> MFQKFISKHNAPINSTQLAATKTPAVAAPVLSVPNLSRSTILINATTTAVTTHSGLCHVVRIDETNPTNHHALSIAGSLSNVPADMIAFAIRFEVADGVVPTAVPALYDVYPIETFNNGKAISF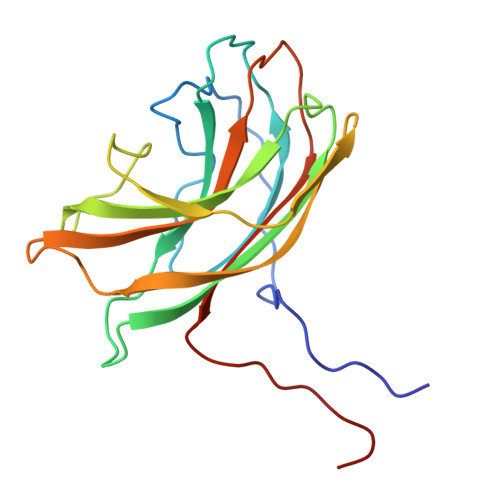KDAVTIDSHPRTVGNDVYAGIMLWSNAWTASTISGVLSVNQVNREATVLQPLK> XLAADLAQA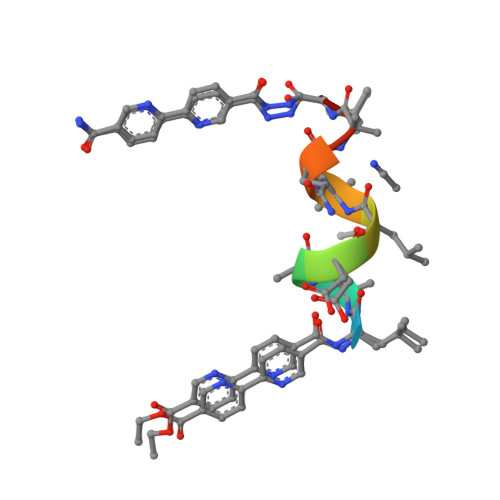LX>[4x]MKGFAMLGINKLGWIEKERPVAGSYDAIVRPLAVSPCTSDIHTVFEGALGDRKNMILGHEAVGEVVEVGSEVKDFKPGDRVIVPCTTPDWRSLEVQAGFQQHSNGMLAGWKFSNFKDGVFGEYFHVNDADMNLA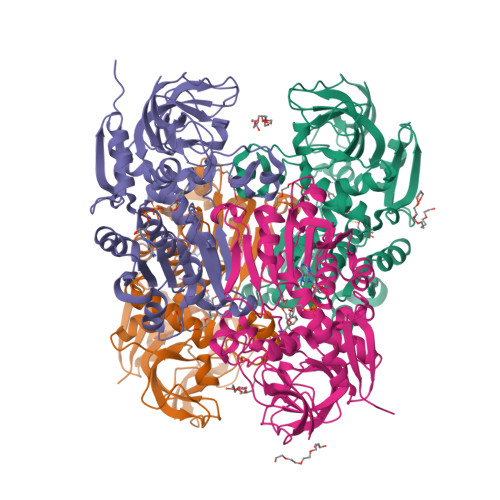ILPKDMPLENAVMITDMMTTGFHGAELADIQMGSSVVVIGIGAVGLMGIAGAKLRGAGRIIGVDYRPICVEAAKFYGATDILNPKNGHIVDQVMKLTNGKGVDRVIMAGGGSETLSQAVSMVKPGGIISNINYHGSGDALLIPRVEWGCGMAHKTIKGGLCPGGRLRAEMLRDMVVYNRVDLSKLVTHVYHGFDHIEEALLLMKDKPKDLIKAVVILHHHH>QGLYVGGFVDVVSCPKLEQELYLDPDQVTDYLPVTEPLPITIEHLPETEVGWTLGLFQVSHGIFCTGAITSPAFLELASRLADTSHVARAPVKNLPKEPLLEILHTWLPGLSLSSIHPRELSQTPSGPVFQHVSLCALGRRRGTVAV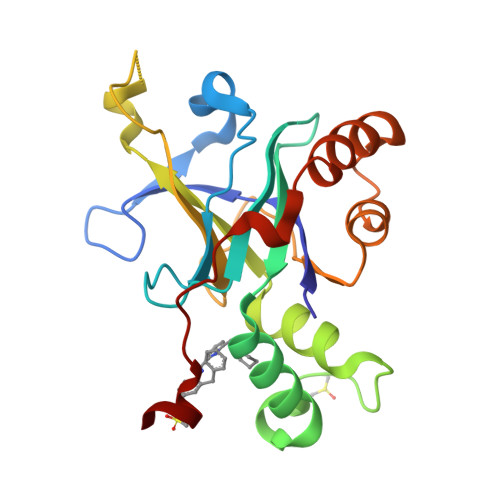YGHDAEWVVSRFSSVSKSERAHILQHVSSCRLEDLSTPNFVSPLETL[2x]>MAGMKTASGDYIDSSWELRVFVGEEDPEAESVTLRVTGESHIGGVLLKIVEQINRKQDWSDHAIWWEQKRQWLLQTHWTLDKYGILADARLFFGPQHRPVILRLPNRRALRLRASFSQPLFQAVAAICRLLSIRHPEELSLLRAPEKKEKKKKEKEPEEELYD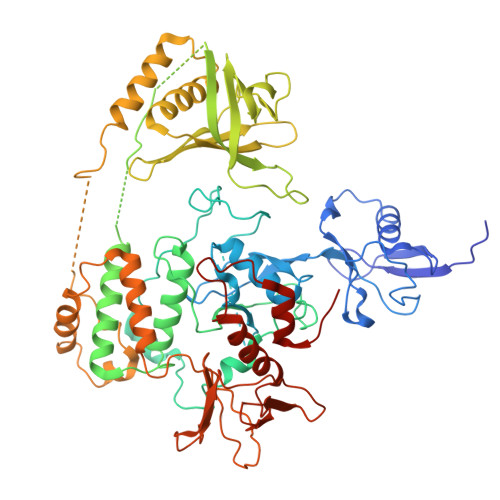LSKVVLAGGVAPALFRGMPAHFSDSAQTEACYHMLSRPQPPPDPLLLQRLPRPSSLSDKTQLHSRWLDSSRCLMQQGIKAGDALWLRFKYYSFFDLDPKTDPVRLTQLYEQARWDLLLEEIDCTEEEMMVFAALQYHINKLSQSGXXXXXXXXXXXXXXXXXXXXXXXXXXXXXXXXXXXXXXXXXPELKDHLRIFRIPRRPRKLTLKGYRQHWVVFKETTLSYYKSQDEAPGDPIQQLNLKGCEVVPDVNVSGQKFCIKLLVPSPEGMSEIYLRCQDEQQYARWMAGCRLASKGRTMADSSYTSEVQAILAFLSLQRTGSGGPGNHPHGPDASAEGLNPYGLVAPRFQRKFKAKQLTPRILEAHQNVAQLSLAEAQLRFIQAWQSLPDFGISYVMVRFKGSRKDEILGIANNRLIRIDLAVGDVVKTWRFSNMRQWNVNWDIRQVAIEFDEHINVAFSCVSASCRIVHEYIGGYIFLSTRERARGEELDEDLFLQLTGGHEAFLEHHHHHH[3x]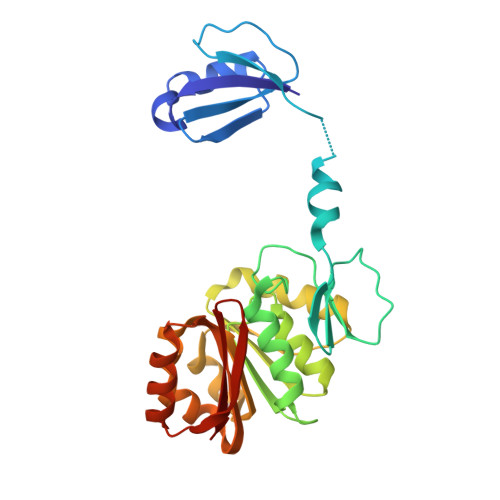> MWVYRLKGTLEALDPILPGLFDGGARGLWEREGEVWAFFPAPVDLPYEGVWEEVGDEDWLEAWRRDLKPALAPPFVVLAPWHTWEGAEIPLVIEPGMAFGTGHHETTRLALKALARHLRPGDKVLDLGTGSGVLAIAAEKLGGKALGVDIDPMVLPQAEANAKRNGVRPRFLEGSLEAALPFGPFDLLVANLYAELHAALAPRYREALVPGGRALLTGILKDRAPLVREAMAGAGFRPLEEAAEGEWVLLAYGR> IKVVIEGKAEDL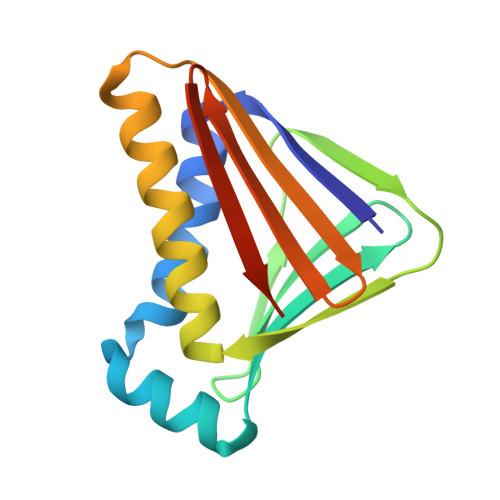LEEMEKIKESLSKFPEEKLKELEKKGYKATIVVKEDGTITVYNELTKEKHTLKKGKVTVEGKGEKKIELPLLTAYKVASDIVETLRKGIEAGATDASITLEYKDGKITITVKVGKLEKTLTVDLEHHHHHH>GQPPPIQLATNYRQDIDVTQYYVSEKLDGIRAYWNGHQLISKQGNIFTAPTWFIASFPTTAMDGELWIARQQFETVSGIARTQDNQNEQWKQIKFMIFDLPKSTVSFEQRINKMQTLVTDTNSPYLQMIEQQKIPNTVAL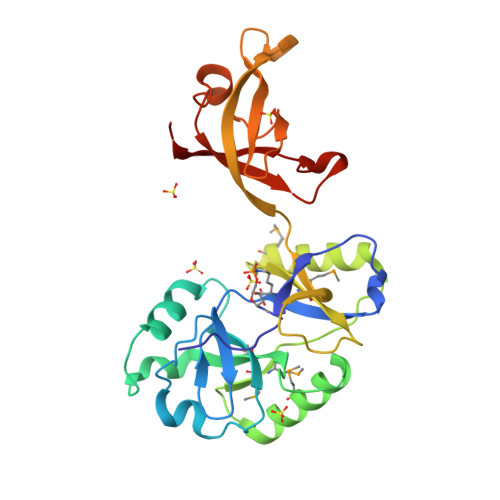FDLLNKVVMGKGEGLMLHHQDALYQTKRSRDLMKLKKFEDAEATVIAYLPGKGKYEGLLGAILVKNEEGVTFKIGSGFSDEERSTPPPIGSLITYRFTGKTNNNIPRFASFVRIRVIY[2x]3,6-Bis{3-(3-[(3R)-methylpiperidino)]propionamido}acridine 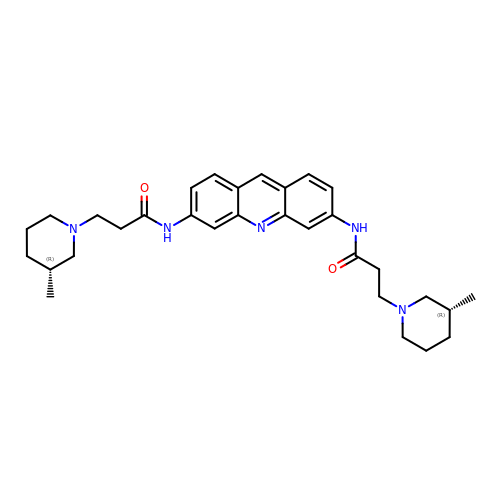| C31 H41 N5 O2 | JGEGKUSUCAFTEW-DHIUTWEWSA-N>[4x]RSSHHHHHHGEFDIPTTENLYFQSGIRRKCPNVLNDPVNVRINCIPEQFPTEGICAQRGCCWRPWNDSLIPWCFFVDNHGYNVQDMTTTSIGVEAKLNRIPSPTLFGNDINSVLFTTQNQTPNRFRFKITDPNNRRYEVPHQYVKEFTGPTVSDTLYDVKVAQNPFSIQVIRKSNGKTLFDTS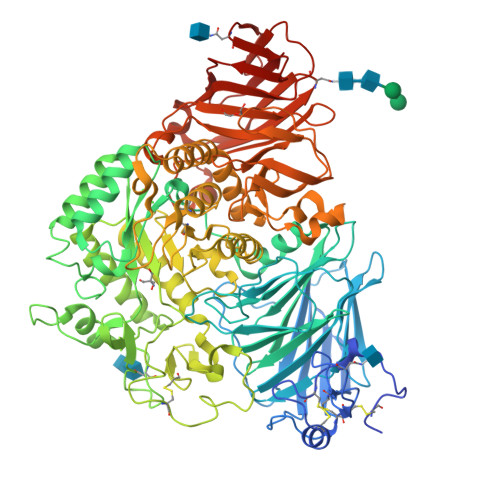IGPLVYSDQYLQISARLPSDYIYGIGEQVHKRFRHDLSWKTWPIFTRDQLPGDNNNNLYGHQTFFMCIEDTSGKSFGVFLMNSNAMEIFIQPTPIVTYRVTGGILDFYILLGDTPEQVVQQYQQLVGLPAMPAYWNLGFQLSRWNYKSLDVVKEVVRRNREAGIPFDTQVTDIDYMEDKKDFTYDQVAFNGLPQFVQDLHDHGQKYVIILDPAISIGRRANGTTYATYERGNTQHVWINESDGSTPIIGEVWPGLTVYPDFTNPNCIDWWANECSIFHQEVQYDGLWIDMNEVSSFIQGSTKGCNVNKLNYPPFTPDILDKLMYSKTICMDAVQNWGKQYDVHSLYGYSMAIATEQAVQKVFPNKRSFILTRSTFAGSGRHAAHWLGDNTASWEQMEWSITGMLEFSLFGIPLVGADICGFVAETTEELCRRWMQLGAFYPFSRNHNSDGYEHQDPAFFGQNSLLVKSSRQYLTIRYTLLPFLYTLFYKAHVFGETVARPVLHEFYEDTNSWIEDTEFLWGPALLITPVLKQGADTVSAYIPDAIWYDYESGAKRPWRKQRVDMYLPADKIGLHLRGGYIIPIQEPDVTTTASRKNPLGLIVALGENNTAKGDFFWDDGETKDTIQNGNYILYTFSVSNNTLDIVCTHSSYQEGTTLAFQTVKILGLTDSVTEVRVAENNQPMNAHSNFTYDASNQVLLIADLKLNLGRNFSVQW> GSAMGQNPWATTTAFADFMKRFNIPQVHGSGIFVDLGRDTEGYREVGGKCPVFGKAIQMHQPAEYSNNFLDDAPTSNDASKKPLPGGFNNPQVYTSGQKFSPIDDSLLQERLGTAGPKTAIGRCALYAYSTIAVNPSTNYTSTYKYPFVYDAVSRKCYVLSVSAQLLKGEKYCSVNGTPSGLTWACFEPVKEKSSARALVYGSAFVAEGNPDAWQSACPNDAVKDALFGKWEDGQCVPFDTKTSV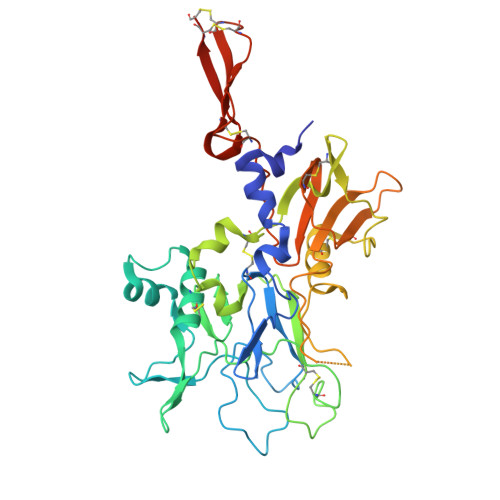QSDQATNKEECWKRVFANPLVASDAPTTYPEAAQKNWNDFWPVHEQSSPKSGGFGANWANFYLEKESGETICAIFDQVPDCFAPITGAVAYTALGSSTEVNLPQCDSASFIPIEGPCNNCVQVVTECVGNQFDQTSKACCTEPEAAALVPR Solution and crystal data are reported for DNA 18-mers with sequences related to those of bacterial noncoding single-stranded DNA segments called repetitive extragenic palindromes (REPs). REPs are DNA segments of about 30 nucleotides in length that occur frequently in some bacterial species. The center of the duplex is formed by two successive T–T mismatches.

In this study, we focus on two REP-related oligonucleotide sequences called Hpar-18 and Chom-18. The crystal structures of all three oligonucleotides, Chom-18, Chom-18Br and Hpar-18, were determined using highly anisotropic data at a relatively low resolution of worse than 2.6 Å. Experimental phasing was necessary because no molecular model was available. The subsequent refinement unequivocally established that all three 18-mers form antiparallel double helices in the crystal phase. The structures are highly similar: the calculated r.m.s.d. between all 365 non-H atoms of Chom-18 and Hpar-18 is 1.0 Å and the r.m.s.d. between Chom-18 and Chom-18Br is 0.24 Å. The crystal structures contain one central and one (in Hpar-18 and Chom-18Br) or two (in Chom-18) peripheral Sr2+ cations. In all three structures the central Sr2+ links the two O4 atoms of the symmetry-related mismatched thymines T9–T9*. In all cases the crystallization solutions contained Na+, a quadruplex-inducing metal, but also the quadruplex-breaking Mg2+ (in Chom-18 and Chom-18Br) and Li+ (in Hpar-18). In both the Chom-18 and Chom-18Br structures, all but two central steps are assigned to NtC classes, while in Hpar-18 two additional steps, 4–5 and 12–13, cannot be assigned and are formally assigned NtC class NANT.

> GGTGGGGCUTGCCCCACC>MLPSAQVARLKPDPFPPSLSPIPHGAVTFAALAPCHNLPIFSSRQMLRDSLTYSHTSPTMSPQIANRFEASLDAQDIARISLFTLESGVILRDVPVAYKSWGRMNVSRDNCVIVCHTLTSSAHVTSWWPTLFGQGRAFDTSRYFIICLNYLGSPFGSAGPCSPDPDAEGQRPYGAKFPRTTIRDDVRIHRQVLDRLGVRQIAAVVGASMGGMHTLEWAFFGPEYVRKIVPIATSCRQSGWCAAWFETQRQCIYDDPKYLDGEYDVDDQPVRGLETARKIANLTYKSKPAMDERFHMAPGVQAGRNISSQDAKKEINGTDSGNSHRAGQPIEAVSSYLRYQAQKFAASFDANCYIAMTLKFDTHDISRGRAGSIPEALAMITQPAL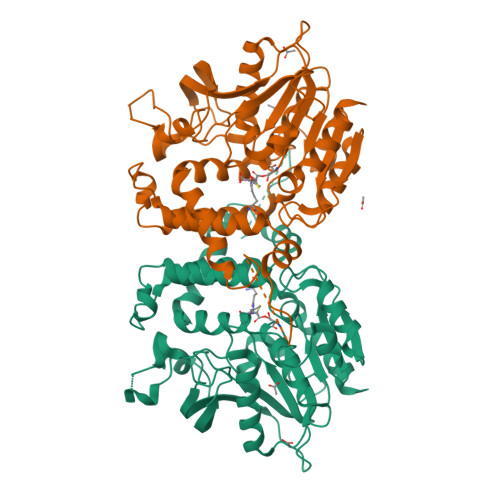IICARSDGLYSFDEHVEMGRSIPNSRLCVVDTNEGHDFFVMEADKVNDAVRGFLDQSLM[12x]> AVEPKEDTITVTAAPAPQESAWGPAATIAARQSATGTKTDTPIQKVPQSISVVTAEEMALHQPKSVKEALSYTPGVSVGTRGASNTYDHLIIRGFAAEGQSQNNYLNGLKLQGNFYNDAVIDPYMLERAEIMRGPVSVLYGKSSPGGLLNMVSKRPTTEPLKEVQFKAGTDSLFQTGFDFSDSLDDDGVYSYRLTGLARSANAQQKGSEEQRYAIAPAFTWRPDDKTNFTFLSYFQNEPETGYYGWLPKEGTVEPLPNGKRLPTDFNEGAKNNTYSRNEKMVGYSFDHEFNDTFTVRQNLRFAENKTSQNSVYGYGVCSDPANAYSKQCAALAPADKGHYLARKYVVDDEKLQNFSVDTQLQSKFATGDIDHTLLTGVDFMRMRNDINAWFGYDDSVPLLNLYNPSSHHHHHHGSSVNTDFDFNAKDPANSGPYRILNKQKQTGVYVQDQAQWDKVLVTLGGRYDWADQESLNRVAGTTDKRDDKQFTWRGGVNYLFDNGVTPYFSYSESFEPSSQVGKDGNIFAPSKGKQYEVGVKYVPEDRPIVVTGAVYNLTKTNNLMADPEGSFFSVEGGEIRARGVEIEAKAALSASVNVVGSYTYTDAEYTTDTTYKGNTPAQVPKHMASL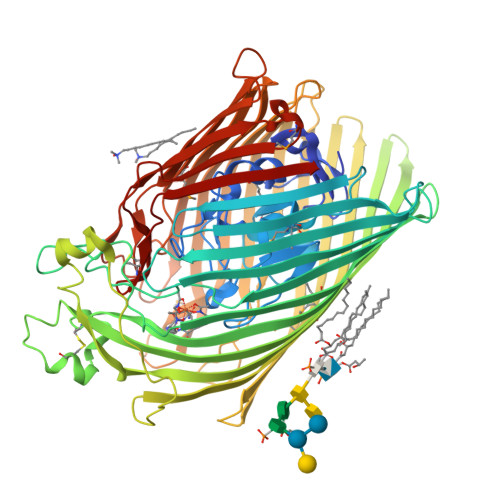WADYTFFDGPLSGLTLGTGGRYTGSSYGDPANSFKVGSYTVVDALVRYDLARVGMAGSNVALHVNNLFDREYVASCFNTYGCFWGAERQVVATATFRF>[6x]MLNQELELSLNMAFARAREHRHEFMTVEHLLLALLSNPSAREALEACSVDLVALRQELEAFIEQTTPVLPASEEERDTQPTLSFQRVLQRAVFHVQSSGRNEVTGANVLVAIFSEQESQAAYLLRKHEVSRLDVVNFISHGTRKDEPTQSSDPGSQPNSEEQAGGEERMENFTTNLNQLARVGGIDPLIGREKELERAIQVLCRRRKNNPLLVGESGVGKTAIAEGLAWRIVQGDVPEVMADCTIYSLDIGSLLAGTKYRGDFEKRFKALLKQLEQDTNSILFIDEIHTIIGAGAASGGQVDAANLIKPLLSSGKIRVIGSTTYQEFSNIFEKDRALARRFQKIDITEPSIEETVQIINGLKPKYEAHHDVRYTAKAVRAAVELAVKYINDRHLPDKAIDVIDEAGARARLMPVSKRKKTVNVADIESVVARIARIPEKSVSQSDRDTLKNLGDRLKMLVFGQDKAIEALTEAIKMARAGLGHEHKPVGSFLFAG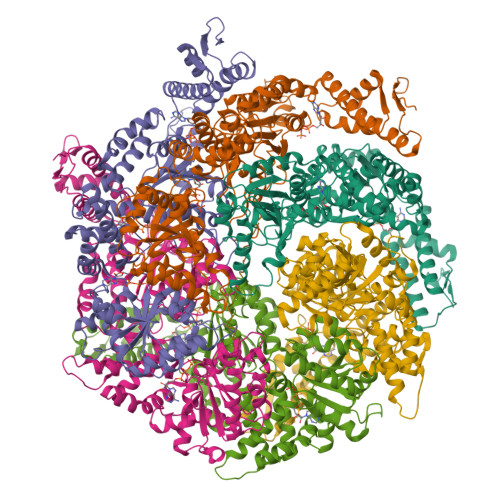PTGVGKTEVTVQLSKALGIELLRFDMSEYMERHTVSRLIGAPPGYVGFDQGGLLTDAVIKHPHAVLLLDEIEKAHPDVFNILLQVMDNGTLTDNNGRKADFRNVVLVMTTNAGVRETERKSIGLIHQDNSTDAMEEIKKIFTPEFRNRLDNIIWFDHLSTDVIHQVVDKFIVELQVQLDQKGVSLEVSQEARNWLAEKGYDRAMGARPMARVIQDNLKKPLANELLFGSLVDGGQVTVALDKEKNELTYGFQSAQKHKAEAAH> MARTKSRKRSGNNQNKNASVVNNKAEIAAMIDARRLEQKKKGGVTNSKGKTNKVVDAKLEKEFKDVLQRFQVQENDTPKEITKDEKNNHVVIVEKNPVMNRKHTAEDELEDTPSDGIEEHLSARKRRKTEKPSLSQLKSQVPYPQIIEWYDCDARYPGLLASIKCTKNVIPVPSHWQSKKEYLSGR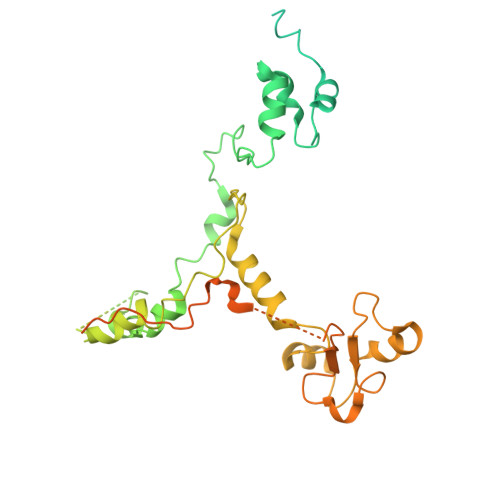SLLGKRPFELPDIIKKTNIEQMRSTLPQSGLDGQDEKSLKEASRARVQPKMGALDLDYKKLHDVFFKIGANWKPDHLLCFGDVYYENRNLFEETNWKRMVDHKRPGRISQELRAIMNLPEGQLPPWCMKMKDIGLPTGYPDLKIAGLNWDITNLKGDVYGKIIPNHHSRSKKQGRNYFGALISFETPEFENSKEDTQANAENGRQDDKIDDEVEHKLDHFQEDISEVTSAEEKLERNEEESEKQLYTVLK Trimeric capsomers of the VACV D13 protein form a transitory, stabilizing lattice on the surface of the initial spherical immature virus particle. The crystal structure of D13 reveals that this major scaffolding protein comprises a double β barrel “jelly-roll” subunit arranged as pseudo-hexagonal trimers. The D13 lattice seems to act as a mechanical scaffold for the growing crescent membrane of the IV with sufficient rigidity to maintain a constant radius of curvature of the crescents even before they close to form complete spheres (Chlanda et al., 2009; Heuser, 2005), thereby fixing the size of the immature virion.

A mutant of D13 with a single amino acid change from aspartic acid to glycine at position 513 (D13D513G) polymerizes into flat sheets of protein composed of hexagonal lattices (Szajner et al., 2005), which do not associate with membrane bilayers but form layered stacks (Szajner et al., 2005), and irregular membranes are formed that lack a D13 scaffold, similar to those seen when the expression of D13 is repressed. The structure of D13D513G was solved by SAD analysis of SeMet-labeled protein crystals, and refined to 3.0 Å resolution with residuals R/Rfree = 0.170/0.203. For the structure of D13D513G at 3.0 Å, density has been attributed to residues Asn2 to Ile10 and modeled (no density is observed between Ile10 and Ser15). Overall the D13D513G mutant is almost identical to the wild-type protein (0.3 Å root-mean-square deviation [rmsd] over 533 Cα atoms). The D513G mutation lies in the H2-I2 loop and the glycine introduces a degree of flexibility to the loop, which adopts three slightly different conformations in the subunits of the D13D513G trimer. The mutated residue, 513 lies in a solvent-accessible position on the outside of the trimer. The orientation of the trimers within the PRD1-derived lattice matches the electron microscopy data and the morphology-modifying residue 513 lies at the interface between neighboring trimers. In addition, the mutant structure contains well-resolved electron density for residues 2–10 at the N terminus of the protein (not observed in the wild-type structure), which form a short α helix that precedes the long N-terminal tail of each subunit. D13D513G and wild-type D13 trimers differ only in the additional short N-terminal helix (residues 2–10) visualized in the structure of D13D513G. This “hook” projects upward from the trimer base and is wedged between the V1 and V2 jelly-rolls of the other two adjacent subunits in the trimer, contributing an extra 1152 Å2 of buried surface area to that subunit interface. In addition to these electrostatic characteristics, the somewhat separate amphipathic N-terminal helix of D13 (residues 2–10, seen in the D13D513G structure) may also stabilize interaction with the membrane by more direct contacts.

>MAHHHHHHSSGLEVLFQGPNNTIINSLIGGDDSIKRSNVFAVDSQIPTLYMPQYISLSGVMTNDGPDNQAIASFEIRDQYITALNHLVLSLELPEVKGMGRFGYVPYVGYKCINHVSISSCNGVIWEIEGEELYNNCINNTIALKHSGYSSELNDISIGLTPNDTIKEPSTVYVYIKTPFDVEDTFSSLKLSDSKITVTVTFNPVSDIVIRDSSFDFETFNKEFVYVPELSFIGYMVKNVQIKPSFIEKPRRVIGQINQPTATVTEVHAATSLSVYTKPYYGNTDNKFISYPGYSQDEKDYIDAYVSRLLDDLVIVSDGPPTGYPESAEIVEVPEDGIVSIQDADVYVKIDNVPDNMSVYLHTNLLMFGTRKNSFIYNISKKFSAITGTYSDATKRTIFAHISHSINIIDTSIPVSLWTSQRNVYNGDNRSAESKAKDLFINDPFIKGIDFKNKTDIISRLEVRFGNDVLYSENGPISRIYNELLTKSNNGTRTLTFNFTPKIFFRPTTITANVSRGKDKLSVRVVYSTMGVNHPIYYVQKQLVVVCNDLYKVSYDQGVSITKIMGDNN[3x]> MTELNSFQTEEITPFGLKITPQYSDQHIDTLPVEQLKELARKHHLLILRGFKSDLSDHEKYEKYARNWGEIMMWPFGAILDVREHQDATDHVFDNSYMPLHWDGMYKPTIPEFIMFHCAHAPESDQGGRTTFVNTRRVVANATQQQLEQWKNISITYRINKVTHYGGEVHSPLVEEHPDRNGFVIRYNEPAVDGEKFLNKHAIEYHNINPDQVAEFQQDFINILYDKRHLYAHAWKKSDLVIVDNFSLLHGREGFTSKSERHLQR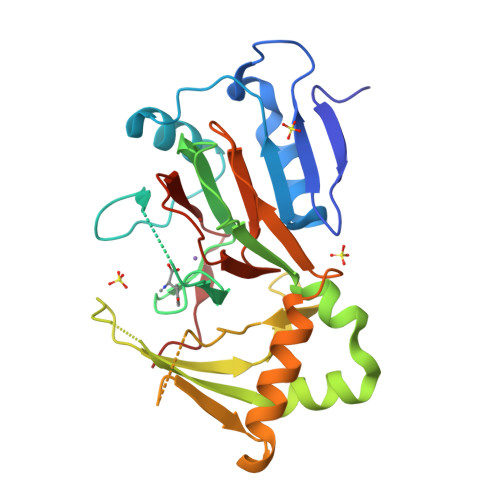IHIQSNPAFNNQALRS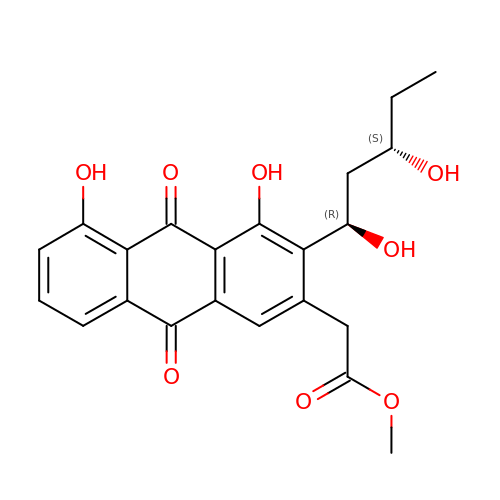{3-[(1R,3S)-1,3-DIHYDROXYPENTYL]-4,5,9,10-TETRAHYDROXY-2-ANTHRYL}ACETATE | C22 H22 O8 | SIHNJMGWRHPFAZ-XHDPSFHLSA-N>[2x]MSDDMSMGLPSSAGEHGVLRSMQEVAMSSQEASKMLRTYNIAWWGNNYYDVNELGHISVCPDPDVPEARVDLAQLVKTREAQGQRLPALFCFPQILQHRLRSINAAFKRARESYGYNGDYFLVYPIKVNQHRRVIESLIHSGEPLGLEAGSKAELMAVLAHAGMTRSVIVCNGYKDREYIRLALIGEKMGHKVYLVIEKMSEIAIVLDEAERLNVVPRLGVRARLASQGSGKWQSSGGEKSKFGLAATQVLQLVETLREAGRLDSLQLLHFHLGSQMANIRDIATGVRESARFYVELHKLGVNIQCFDVGGGLGVDYEGTRSQSDCSVNYGLNEYANNIIWAIGDACEENGLPHPTVITESGRAVTAHHTVLVSNIIGVERNEYTVPTAPAEDAPRALQSMWETWQEMH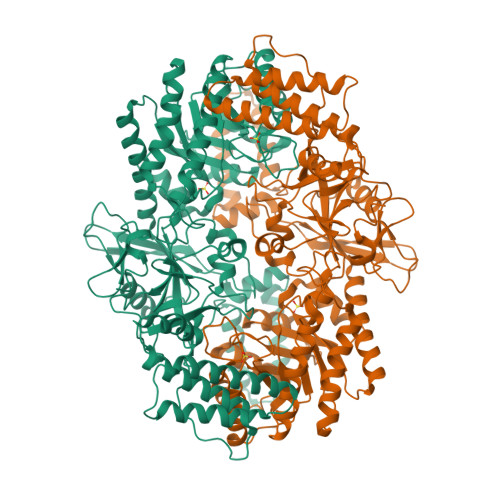EPGTRRSLREWLHDSQMDLHDIHIGYSSGIFSLQERAWAEQLYLSMCHEVQKQLDPQNRAHRPIIDELQERMADKMYVNFSLFQSMPDAWGIDQLFPVLPLEGLDQVPERRAVLLDITCDSDGAIDHYIDGDGIATTMPMPEYDPENPPMLGFFMVGAYQEILGNMHNLFGDTEAVDVFVFPDGSVEVELSDEGDTVADMLQYVQLDPKTLLTQFRDQVKKTDLDAELQQQFLEEFEAGLYGYTYLEDELEHHHHHH>MKGLVELGEKAPDFTLPNQDFEPVNLYEVLKRGRPAVLIFFPA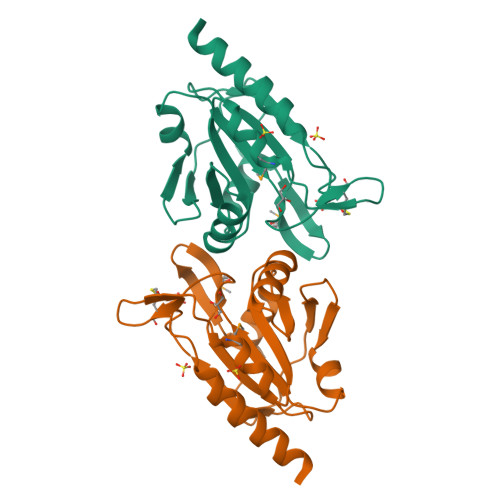AFSPVCTKELCTFRDKMAQLEKANAEVLAISVDSPWCLKKFKDENRLAFNLLSDYNREVIKLYNVYHEDLKGLKMVAKRAVFIVKPDGTVAYKWVTDNPLNEPDYDEVVREANKIAGELVA[2x]>GASLAQPPLPVLPPFPPPSGKNPVMILNELRPGLKYDFLSESGESHAKSFVMSVVVDGQFFEGSGRNKKLAKARAAQSALAAIFNLHLDQTPSRQPIPSEGLQLHLPQVLADAVSRLVLGKFGDLTDNFSSPHARRKVLAGVVMTTGTDVKDAKVISVSTGTKCINGEYMSDRGLALNDCHAEIISRRSLLRFLYTQLELYLNNKDDQKRSIFQKSERGGFRLKENVQFHLYISTSPCGDARIFSPHEPILEEPADRHPNRKARGQLRTKI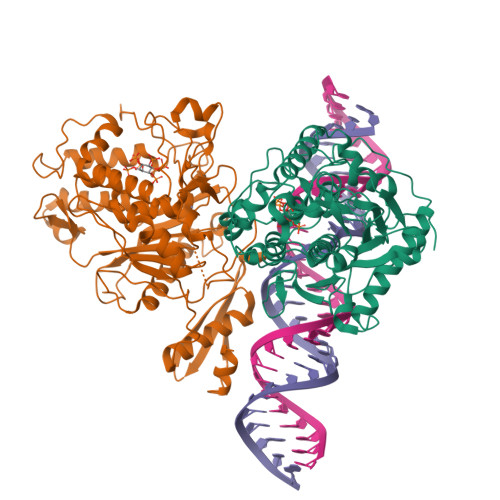ESGQGTIPVRSNASIQTWDGVLQGERLLTMSCSDKIARWNVVGIQGSLLSIFVEPIYFSSIILGSLYHGDHLSRAMYQRISNIEDLPPLYTLNKPLLSGISNAEARQPGKAPNFSVNWTVGDSAIEVINATTGKDELGRASRLCKHALYCRWMRVHGKVPSHLLRSKITKPNVYHESKLAAKEYQAAKARLFTAFIKAGLGAWVEKPTEQDQFSLTP[2x]>MDKAKRNIKPFDGEKYAIWKFRIRALLAEQDVLKVVDGLMPNEVDDSWKKAE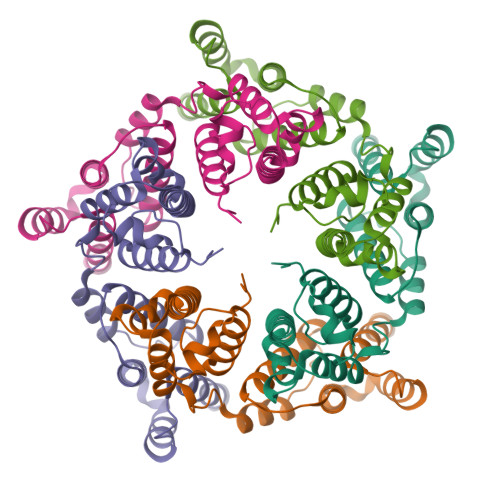RCAKSTIIEYLSDSFLNFATSDITARQILENLDAVYERKSLASQLALRKRLLSLKLSSEMSLLSHFHIFDELISELLAAGAKIEEMDKISHLLITLPSCYDGIITAIETLSEENLTLAFVKNRLLDQEIKIKNDHNDTSKKVMNAIVHNNNNTYKNNLFKNRVTKPKKIFKGNSKYKVKCHHCGREGHIKKDCFHYKRILNNKNKENEKQVQTATSHG[5x]>MGHMNITDIREQFPILHQQVNGHDLVYLDSAATSQKPRAVIETLDKYYNQYNSNVHRGVHTLGTRATDGYEGAREKVRKFINAKSMAEIIFTKGTTTSLNMVALSYARANLKPGDEVVITYMEHHANIIPWQQAVKATGATLKYIPLQEDGTISLEDVRETVTSNTKIVAVSHVSNVLGTVNPIKEMAKIAHDNGAVIVVDGAQSTPHMKIDVQDLDCDFFALSSHKMCGPTGVGVLYGKKALLENMEPAEFGGEMIDFVGLYESTWKELPWKFEAGTPIIAGAIGLGAAIDFLEEIGLDEISRHEHKLAAYALERFRQLDGVTVYGPEERAGLVTFNLDDVHPHDVATVLDAEGIAVRAGHHCAQPLMKWLDVTATARASFYLYNTEEEIDKLVEALQKTKEYFTNVFVDLEHHHHHH[2x];>[2x]MSFNANLDTLYRQVIMDHYKNPRNKGVLNDSIVVDMNNPTCGDRIRLTMKLDGDIVEDAKFE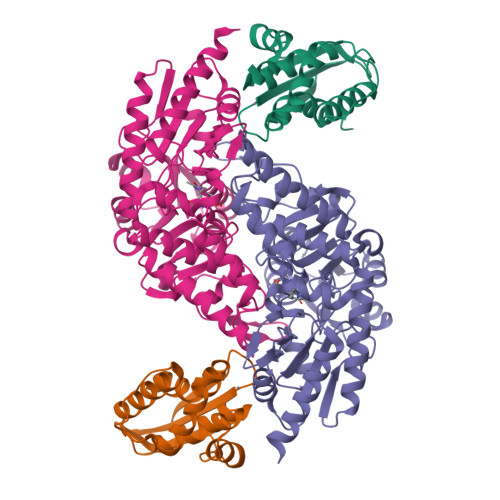GEGCSISMASASMMTQAIKGKDIETALSMSKIFSDMMQGKEYDDSIDLGDIEALQGVSKFPARIKCATLSWKALEKGVAKEEGGNLEHHHHHH4-(3-methyl-4-oxidanyl-phenyl)quinolin-7-ol | C16 H13 N O2 | 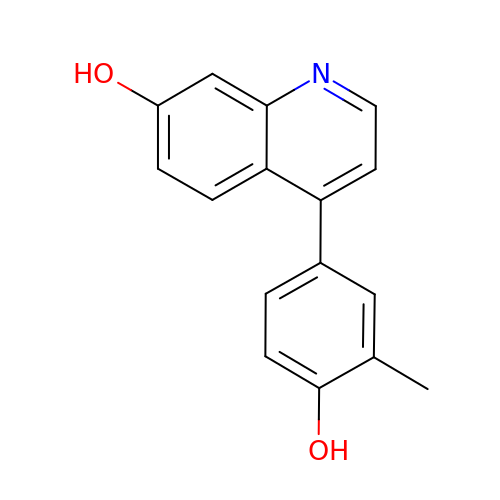QXFYDRYRLOHSBD-UHFFFAOYSA-N>[2x]GLQGTENLYFQSHMTIAVTGSIATDHLMRFPGRFSEQLLPEHLHKVSLSFLVDDLVMHRGGVAGNMAFAIGVLGGEVALVGAAGADFADYRDWLKARGVNCDHVLISETAHTARFTCTTDVDMAQIASFY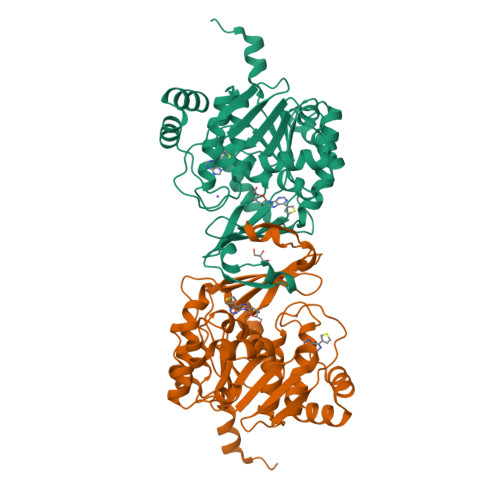PGAMSEARNIKLADVVSAIGKPELVIIGANDPEAMFLHTEECRKLGLAFAADPSQQLARLSGEEIRRLVNGAAYLFTNDYEWDLLLSKTGWSEADVMAQIDLRVTTLGPKGVDLVEPDGTTIHVGVVPETSQTDPTGVGDAFRAGFLTGRSAGLGLERSAQLGSLVAVLVLESTGTQEWQWDYEAAASRLAGAYGEHAAAEIVAVLA4-[2-azanyl-8-[[(2~{S})-1-oxidanylpropan-2-yl]amino]quinazolin-6-yl]-5-ethyl-2-fluoranyl-phenol 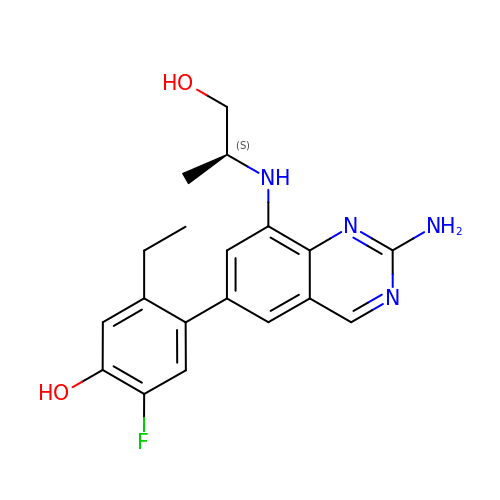| C19 H21 F N4 O2 | LICCUQPKNWSBNT-JTQLQIEISA-N> APTSSSTKKTQLQLEHLLLDLQMILNGINNYKNPKLTRMLTFKFYMPKKATELKHLQCLEEELKKLEEVLNLAQSKNFHLRPRDLISNINVIVLELKGSETTFMCEYADETATIVEFLNRWITFSQSIISTLT

IL-2 functions as a lymphocyte growth and stimulatory factor, signaling via activation of the heterodimeric IL-2 receptor complex consisting of two subunits, IL-2 receptor β (CD122) and the common γ receptor subunit (CD132), or the heterotrimeric IL-2 receptor complex that includes IL-2 Rα (CD25). IL-2 activation of the IL-2 Rβγ complex induces proliferative and activation signals through STAT5 phosphorylation that drive effector T and natural killer (NK) cell expansion and tumor clearance. In addition to the IL-2 Rβ and γ subunits, certain cell types express the IL-2 Rα subunit, which functions to increase affinity and capture of IL-2 by the signaling complex. Structures of the IL-2/heterotrimeric receptor signaling complex demonstrated that the IL-2 Rα and βγ subunits engage IL-2 from opposite sides and that the α subunit engages IL-2 independently of the IL-2R βγ interfaces.

The IL-2 compound with residue Pro65 replaced with AzK and pegylated with a 30 kDa mPEG, hereafter referred to as THOR-707, exhibited higher expression levels of the precursor protein and was selected for further characterization. The proline residue at position 65 in human IL-2 appears to impart a significant bend in helix H3, a region that mediates substantial interactions with IL-2 Rα14,15. As the sequence of THOR-707 contains a substitution of this proline to a lysine-like residue, we reasoned that this modification might result in a distinct helical conformation that mis-aligns residues critical for IL-2 Rα engagement. To elucidate the tertiary structure of the THOR-707 protein component, the crystal structure of the human IL-2 variant P65K was solved at 1.8 Å resolution. The lysine residue incorporated at position 65 was selected to mimic the effect of the AzK substitution of this position on protein structure, as lysine constitutes the majority of the backbone of the AzK residue without the excessive hydrophobicity of the un-conjugated azide. Surprisingly, the structure of the IL-2 P65K was remarkably similar to that of rhIL-2. Structural alignments show that the lysine substitution for proline at position 65 did not result in large-scale changes to the IL-2 tertiary structure, including the conformation of helix H3. Consistent with the above biochemical and ex vivo data, an inspection of the P65K region in the structure shows that this modification occupies a region of the IL-2/IL-2 Rα interface that mediates productive interactions. The similar stepwise and minor reductions in potency of PEG size variants in both CD8+ T cells and Tregs suggest that PEG polymers are not specifically required to prevent IL-2 Rα engagement, but may impact potency in THOR-707 via non-specific envelopment as observed with other pegylated cytokines. Together, these results suggest that steric effects mediated largely by the substitution of proline 65 with AzK result in the reduction in IL-2 Rα engagement by THOR-707.>ESMELACPAERSGHVAVSDGRHMFVWGGYKSNQVRGLYDFYLPREELWIYNMETGRWKKINTEGDVPPSMSGSCAVCVDRVLYLFGGHHSRGNTNKFYMLDSRSTDRVLQWERIDCQGIPPSSKDKLGVWVYKNKLIFFGGYGYLPEDKVLGTFEFDETSFWNSSHPRGWNDHVHILDTETFTWSQPITTGKAPSPRAAHACATVGNRGFVFGGRYRDARMNDLHYLNLDTWEWNELIPQGICPVGRSWHSLTPVSSDHLFLFGGFTTDKQPLSDA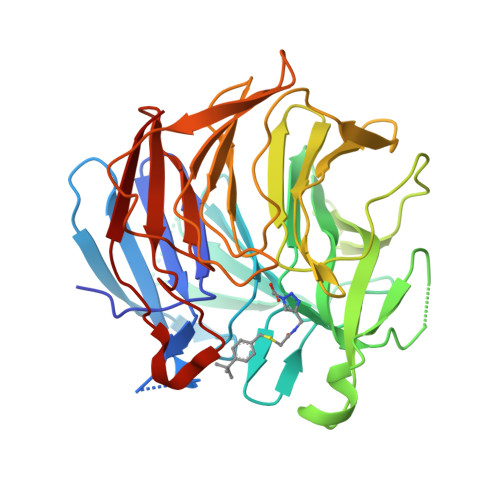WTYCISKNEWIQFNHPYTEKPRLWHTACASDEGEVIVFGGCANNLLVHHRAAHSNEILIFSVQPK[2x]4-(4-tert-butylphenyl)-4-oxobutanoic acid | C14 H18 O3 | 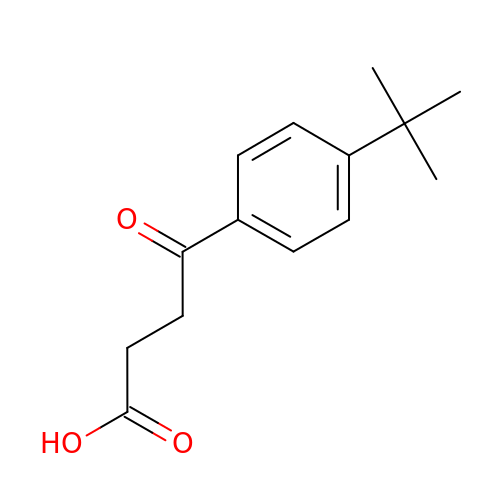XJHBTHNAMOUNRQ-UHFFFAOYSA-N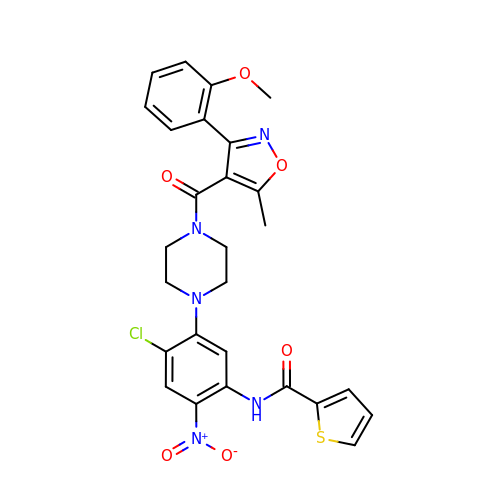N-[4-chloranyl-5-[4-[[3-(2-methoxyphenyl)-5-methyl-1,2-oxazol-4-yl]carbonyl]piperazin-1-yl]-2-nitro-phenyl]thiophene-2-carboxamide | C27 H24 Cl N5 O6 S | HDEDVIXSWBFUIT-UHFFFAOYSA-N We show that lipoteichoic acids (LTAs) but not wall teichoic acids are D-alanylated in Lactiplantibacillus plantarumNC8 cell envelope and demonstrate that DltE is a D-Ala carboxyesterase removing D-Ala from LTA. (a) The dltE gene encodes for a 397 residues protein composed of a transmembrane segment predicted between residues 12 and 34 and a larger C-terminal extracellular region from residues 34–397 and named DltEextra. The domain consists of two subdomains, an α-β sandwich (residues 76–126 and 246–397) that form a five strand (β1–β5) antiparallel β-sheet flanked by 5 α-helices (α2, α9–α12) and an α-helix-rich region (residues 127–245) folding in 6 α-helices (α3-α8). DltE is structurally homologous to the D-Ala-D-Ala carboxypeptidase R61 (DDCP) from Streptomyces (Kelly et al., 1986; McDonough et al., 2002) that exhibits the classical β-lactamase fold of PBPs.

Besides the apo form structure, we obtained two other DltE structures in complex with tartrate or TCEP (Tris(2-carboxyethyl)phosphine hydrochloride), two compounds arising from the crystallization conditions. Intriguingly, these two molecules are anchored by an interaction network that involves eight different residues, among which are the conserved active site nucleophile Ser128 and the base Tyr213 (Ser 62 and Tyr 159 in DDCP). Importantly, the catalytic Ser128 with the hydroxyl group of its side chain positioned at only 2.7 Å away from a carboxylic group of TCEP and tartrate is ideally placed as it would activate a substrate for the enzyme acylation event as described for DDCP. This suggests that the tartrate and TCEP molecule may mimic the nature and position of the natural substrate of DltE in its active site and that the acylation/deacylation step of the catalytic reaction is probably preserved in DltE. Three additional interactions specific to DltE are observed in the TCEP-bond structure and involved Tyr211, Arg345, and Gln381. Notably, a Tyr residue (Tyr338 in DltE) interacting with TCEP or tartrate replaces the conserved arginine (Arg285 in DDCP) in carboxypeptidases. This arginine is key for the recognition of the terminal carboxylate of the peptide substrate and the carboxypeptidase activity (McDonough et al., 2002). Instead, residues specific to DltE (Tyr338, His347, Arg345, and Leu349) stabilize the TCEP or tartrate molecules. Taken collectively, our structural data suggest that DltE would not be able to recognize the D-Ala-D-Ala terminal end of a stem peptide as DDCP does and that DltE would not be a DD-carboxypeptidase.

>[4x]MATERQAAIAKKRQTDKALNKKAALKNSQLSRKINQTTFSNNKNTDEQVTKALNLSHFVGSALVVKNDHVIYNRAFGYANKAKNQRNKVNSKYQILSIQKSMTAVGIMQLVQAGKVKLTDPISKYYPTLKHGRQTTLRQMLDMTTGFRLKSGSKEFLPENQVIDFAAHNVFYYPDKNGIYNYSSVNFLLLAGIIRKVTGQSYQHFFTTHFIDKLNLNETGFLIHGQGQDATTGYRALADQTLPNYDQTMPESKSQMANELGTGQVYMSTADLFTVESAILKGQLLSKKNVAILHTRTATGEYGGGVYNMSNGIRSHGLGYGYESSIFLSPDGKTGVVLMSNYYRKAAGIQATANKIFTELMKGDIKLEHHHHHH> SRHSCIF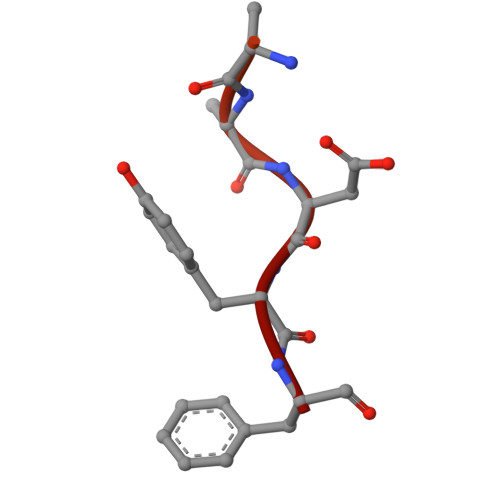PGQYNPSFISDESRRRDYF>[2x]AEFKHVFVCVQDRPPGHPQGSCAQRGSREVFQAFMEKIQTDPQLFMT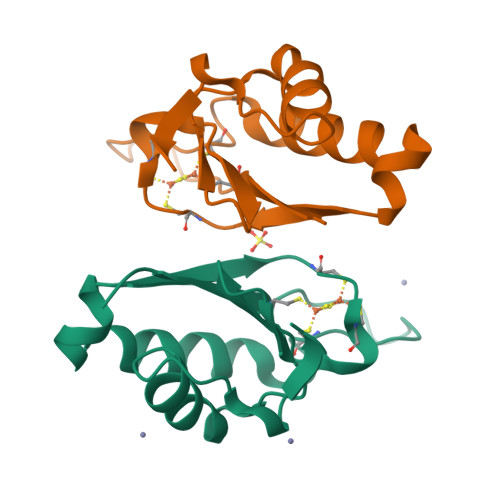TVITPTGCMNACMMGPVVVVYPDGVWYGQVKPEDVDEIVEKHLKGGEPVERLVISKGKPPGMF>[2x]GAGUAGAAGCGUUCAGCGGCCGAAAGGCCGCCCGGAAAUUGCUCC

Very recently, an orphan RNA motif called NMT1 present in proteobacteria was identified to bind xanthine which is an oxidization product generated during purine degradation in purine metabolism. Bacterial RNAs containing the NMT1 motif turn off gene expression upon ligand sensing, likely by regulating translation initiation. Members of this riboswitch class respond to high concentrations of oxidized purines and they regulate genes predominantly associated to purine transport and oxidation, thus avoiding the deleterious effects of accumulation of purine degradation products in the cell. Overall, the riboswitch exhibits a rod-like, continuously stacked fold composed of three stems and two internal junctions.

We screened a large number of in vitro transcribed RNA constructs for crystallization in the presence of xanthine and obtained crystals for a 46 nucleotide long RNA with the sequence from Ideonella species that diffracted to 2.7 Å. In this construct, the variable loop that closes stem P2b was replaced by the extra-stable tetranucleotide loop GAAA to facilitate crystallization. We solved the structure with single-wavelength anomalous diffraction (SAD) phasing by collecting the anomalous signal from Ir(NH3)63+-soaked crystals.Human NAD-IDH is a key enzyme in the TCA cycle, which catalyzes the oxidative decarboxylation of ICT into α-KG. The α and β subunits form a heterodimer (αβ), and the α and γ subunits form another heterodimer (αγ), which are assembled into a heterotetramer (α2βγ) and further into a heterooctamer (the heterotetramer and heterooctamer are also called holoenzyme). Our previous biochemical studies demonstrated that the αγ heterodimer alone exhibits a high enzymatic activity and kinetic properties comparable with those of the holoenzyme and can be activated by CIT and ADP but inhibited by NADH; on the other hand, the αβ heterodimer alone exhibits a low activity and cannot be activated by the activators but can be inhibited by NADH. Our structural comparisons show that the αβ heterodimer has a similar yet more compact overall structure compared with the αγ heterodimer and contains a pseudo-allosteric site that exhibits substantial conformational differences from the allosteric site in the αγ heterodimer.

Crystals of the αβ heterodimer with the α subunit in apo form (αβ) grew at condition I and belong to space group C2, and the structure was determined at 3.06 Å resolution with each asymmetric unit containing eight αβ molecules, which form four dimers of heterodimers via the clasp domains. In this structure, there is no metal ion or ligand bound at the active site. In the αβ and αCaβ structures, most residues of the two subunits are well-defined except the β2-α2 loop (residues 52–60) and the β3-α3 loop (residues 80–93) of the β subunit and a few residues at the N and C termini of the α and β subunits. In the αβ structure, the key residues at the pseudo-allosteric site, the heterodimer interface, and the active site assume similar conformations and form hydrogen-bonding interactions comparable with those in the αCaβ structure, indicating that the αβ structure also exhibits an active overall conformation (data not shown). Similarly, in the αβ structure, Asp-230A, Asp-234A, and Asp-217B assume positions comparable with those in the αCaβ structure and are not in proper positions or conformations to bind the metal ion effectively. Structural analyses suggest that the active overall conformation of the αβ and αCaβ structures could be attributed to the changes of some residues at the pseudo-allosteric site and a unique hydrogen-bonding network, which stabilize the side chain of Tyr-137B and the β5B-β6B loop in the active conformations and further trigger the conformational changes of the heterodimer interface and the active site.

>GSTGGVQTVTLIPGDGIGPEISAAVMKIFDAAKAPIQWEERNVTAIQGPGGKWMIPSEAKESMDKNKMGLKGPLKTPIAAGHPSMNLLLRKTFDLYANVRPCVSIEGYKTPYTDVNIVTIRENTEGEYSGIEHVIVDGVVQSIKLITEGASKRIAEFAFEYARNNHRSNVTAVHKANIMRMSDGLFLQKCREVAESCKDIKFNEMYLDTVCLNMVQDPSQFDVLVMPNLYGDILSDLCAGLIGGLGVTPSGNIGANGVAIFESVHGTAPDIAGKDMANPTALLLSAVMMLRHMGLFDHAARIEAACFATIKDGKSLTKDLGGNAKCSDFTEEICRRVKDLD[8x];>ASRSQAEDVRVEGSFPVTMLPGDGVGPELMHAVKEVFKAAAVPVEFQEHHLSEVQNMASEEKLEQVLSSMKENKVAIIGKIHTPMEYKGELASYDMRLRRKLDLFANVVHVKSLPGYMTRHNNLDLVIIREQTEGEYSSLEHESARGVIECLKIVTRAKSQRIAKFAFDYATKKGRGKVTAVHKANIMKLGDGLFLQCCEEVAELYPKIKFETMIIDNCCMQLVQNPYQFDVLVMPNLYGNIIDNLAAGLVGGAGVVPGESYSAEYAVFETGARHPFAQAVGRNIANPTAMLLSASNMLRHLNLEYHSSMIADAVKKVIKVGKVRTSDMGGYATCHDFTEEICRRVKDLDENLYFQ[8x]>[2x]VSIWSRVVQFGTGWGFWVSGHVFITAKHVAPPKGTEIFGRKPGDFTVTSSGDFLKYYFTSAVRPDIPAMVLENGCQEGVVASVLVKRASGEMLALAVRMGSQ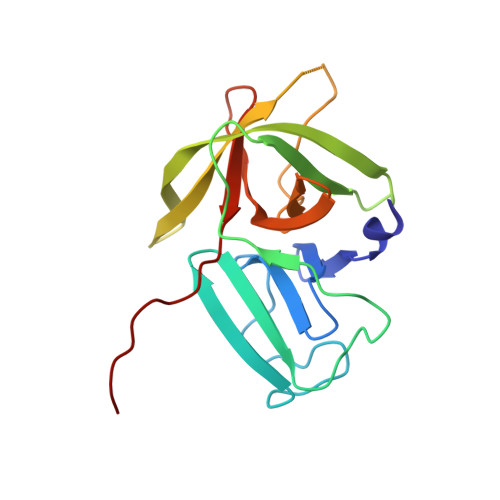AAIKIGSAVVHGQTGMLLTGSNAKAQDLGTIPGDAGCPYVYKKGNTWVVIGVHVAATRSGNTVIAATHGEPTLEALE Among them, one gene codes for a eugenol oxidase (EUGO) that displays significant sequence identity with VAO (≈40 %) and a similar but not fully overlapping pattern of substrate preferences. In addition to the oxidation of vanillyl alcohol and the hydroxylation of eugenol, EUGO can efficiently catalyze the dehydrogenation of various phenolic ketones and the selective oxidation of a racemic secondary alcohol—4‐(1‐hydroxyethyl)‐2‐methoxyphenol. The overall structure of EUGO is highly similar to that of VAO, as indicated by a 1.1 Å rmsd for 490 Cα atom pairs (45 % sequence identity). As predicted, EUGO also shares with VAO the presence of a characteristic covalent bond between His390 (equivalent to His422 of VAO) and the C8M atom of the flavin ring.

The structural bases of substrate and inhibitor binding by the cavity were explored by solving the crystal structures of EUGO in complexes with isoeugenol (inhibitor), coniferyl alcohol (2, reaction product and inhibitor), and vanillin (4, reaction product); these were obtained by crystal soaking, resulting in highly defined electron density maps. All these ligands bind with their aromatic moiety stacking against the pyrimidine ring of the flavin and the Cα atom of the aliphatic substituent lying right above the flavin N5 atom at a distance of 3.2 Å. In this orientation, the ligand 4‐hydroxy group is H‐bonded to Tyr91 and Tyr471 and is also in close contact with Arg472 (3.5 Å). However, comparative analysis of the three‐dimensional structures also revealed striking differences between EUGO and VAO. Above all, inhibitor/product binding differs in a 180° flipped orientation. This can be visualized by superimposing the isoeugenol complexes of the two enzymes. The ligand methoxy groups are in opposed orientations and occupy different niches in the active sites of the two enzymes. In EUGO, the methoxy moiety is in close contact with Gly392, which replaces the Phe424 residue of VAO. This bulkier aromatic side chain of VAO likely creates steric hindrance, impeding the binding orientation found in EUGO. Conversely, the flipped isoeugenol bound to VAO positions the methoxy group in direct contact with a valine residue that is conserved in EUGO (Val166).

>MTRTLPPGVSDERFDAALQRFRDVVGDKWVLSTADELEAFRDPYPVGAAEANLPSAVVSPESTEQVQDIVRIANEYGIPLSPVSTGKNNGYGGAAPRLSGSVIVKTGERMNRILEVNEKYGYALLEPGVTYFDLYEYLQSHDSGLMLDCPDLGWGSVVGNTLDRGVGYTPYGDHFMWQTGLEVVLPQGEVMRTGMGALPGSDAWQLFPYGFGPFPDGMFTQSNLGIVTKMGIALMQRPPASQSFLITFDKEEDLEQIVDIMLPLRINMAPLQNVPVLRNIFMDAAAVSKRTEWFDGDGPMPAEAIERMKKDLDLGFWNFYGTLYGPPPLIEMYYGMIKEAFGKIPGARFFTHEERDDRGGHVLQDRHKINNGIPSLDELQLLDWVPNGGHIGFSPVSAPDGREAMKQFEMVRNRANEYNKDYAAQFIIGLREMHHVCLFIYDTAIPEAREEILQMTKVLVREAAEAGYGEYRTHNALMDDVMATFNWGDGALLKFHEKIKDALDPNGIIAPGKSGIWSQRFRGQNL[2x]> MKKSYLLAALIFFLAGLLHGT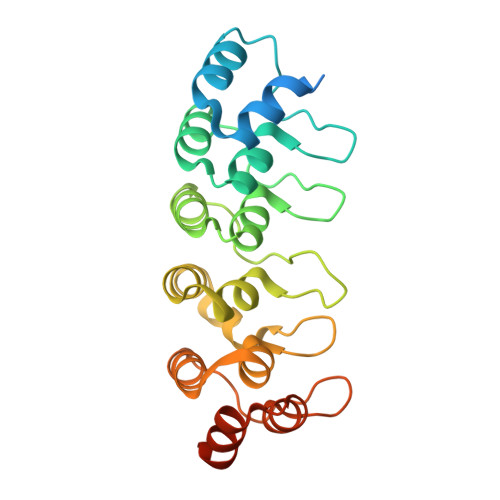AFAMSGKSSKALNEAAEQGDLAKVKNLVQKNKIDLNAQDETGMTPLMNAAMGGNLDIVKFLLSKKVNLELKNNGGETALAFAVTNDAYDVAEELIKAGANVDIIVAGDEGDTLFMRAAQNNKKTAESILAKNKSLINKANTLGETALFAVARYGTPADIDFLIKKGADLKLKNKKGQTALDVAKEASNQDTAKALSKKKLEHHHHHHHH2-{5-[AMINO(IMINIO)METHYL]-1H-BENZIMIDAZOL-2-YL}-4-FLUOROBENZENOLATE | C14 H11 F N4 O | 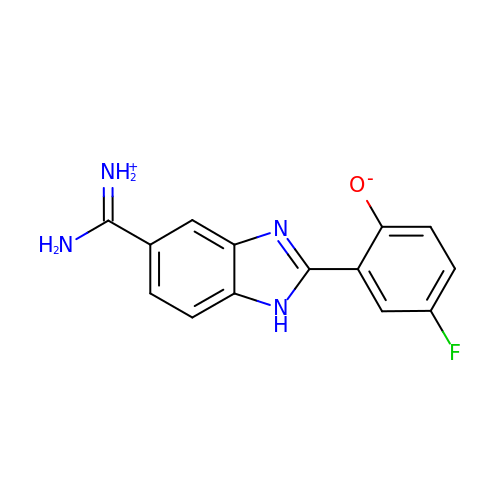JOGOACSSLJEREC-UHFFFAOYSA-N> MSTENPQPLWQPDAQRIAQARITRFQAWAAEHHGAPAEGGYAALHRWSVDELDTFWKAVTEWFDVRFSTPYARVLGDRTMPGAQWFPGATLNYAEHALRAAGTRPDEPALLYVDETHEPAPVTWAELRRQVASLAAELRALGVRPGDRVSGYLPNIPQAVVALLATAAVGGVWTSCAPDFGARSVLDRFQQVEPVVLFTVDGYRYGGKEHDRRDTVAELRRELPTLRAVIHIPLLGTEAPDGT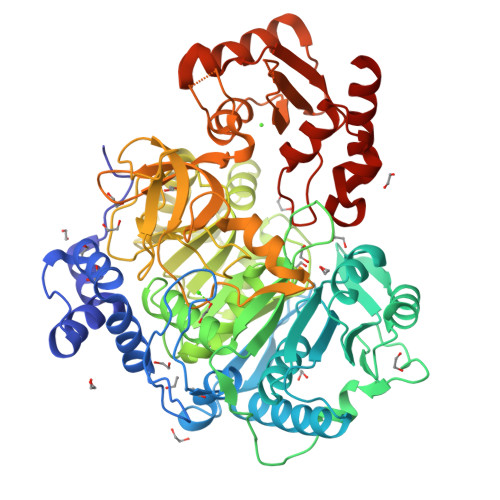LDWETLTAADAEPVYEQVPFDHPLWVLYSSGTTGLPKAIVQSQGGILVEHLKQLGLHCDLGPGDRFFWYTSTGWMMWNFLVSGLLTGTTIVLYDGSPGFPATDAQWRIAERTGATLFGTSAAYVMACRKAGVHPARDLDLSAIQCVATTGSPLPPDGFRWLHDEFAAGGADLWIASVSGGTDVCSCFAGAVPTLPVHIGELQAPGLGTDLQSWDPSGDPLTDEVGELVVTNPMPSMPIRFWNDPDGSRYHDSYFDTYPGVWRHGDWITLTSRGSVVIHGRSDSTLNRQGVRMGSADIYEAVERLPEIRESLVIGIEQPDGGYWMPLFVHLAPGATLDDALLDRIKRTIRVNLSPRHVPDEVIEVPGIPHTLTGKRIEVPVKRLLQGTPLDKAVNPGSIDNLDLLHFYEELARKRS> SDEFDALRIKWATLLTGGPALDPADSDIAARTDKLAQDANDYWEDMDLSSSRTYIWYALRGNGTSDNVNAVYERLRTMALAATTVGSSLYGNADLKEDILDALDWLYVNSYNSTRSRSAYNWWHWQLGIPMSLNDIAVLLYDDISAARMATYMDTIDYFTPSIGLTGAARAWQAIVVGVRAVIVKDAVKLAAARNGLSGTGIFPYATGGDGFYADGSFVQHTTFAYTGGYGSSVLETTANLMYLLSGSTWSVSDPNQSNVWQWIYEAYRPLLYKGAMMDMVRGREISRSYAQDHAVGHGIVASIVRLAQFAPAPH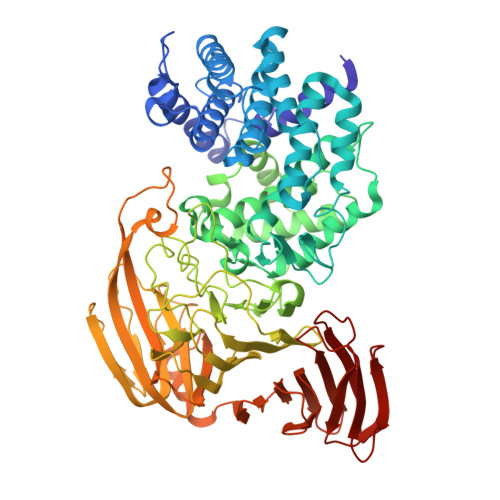AAAFKQIAKRVIQEDTFSSFYGDVSTDTIRLAKAIVDDPSIAPAAAPNLYKQYAAMDRAVLQRPGFALGLALYSTRISSYESINSENGRGWYTGAGATYLYNQDLAQYSEDYWPTVDAYRIPGTTVASGTPIASGTGTSSWTGGVSLAGQYGASGMDLSYGAYNLSARKSWFMFDDEIVALGSGISSTAGIPIETVVDNRKLNGAGDNAWTANGAALSTGLGVAQTLTGVNWVHLAGNTADGSDIGYYFPGGATLQTKREARTGTWKQINNRPATPSTAVTRNYETMWIDHGTNPSGASYGYVLLPNKTSAQVGAYAADPAIEIVVNTSGVQSVKEKTLGLVGANFWTDTTQTADLITSNKKASVMTREIADERLEASVSDPTQANNGTIAIELARSAEGYSADPGITVTQLAPTIKFTVNVNGAKGKSFHASFQLG methylammonium ion | C H6 N | 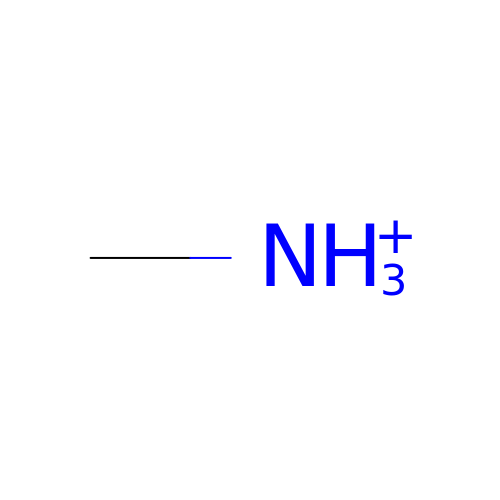BAVYZALUXZFZLV-UHFFFAOYSA-O> GTSSMGYLMALFEDIQAVIAEQLNVDAAQVTPEAE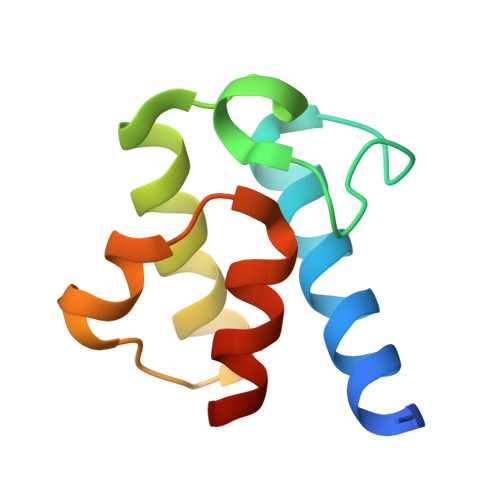FVKDLGADSLDVVELIMALEEKFGIEIPDEQAEKIVNVGDVVKYIEDNKLA>[2x]MSLAKNIVFIGFMGSGKSTLARALAKDLDLVFLDSDFLIEQKFNQKVSEIFEQKRENFFR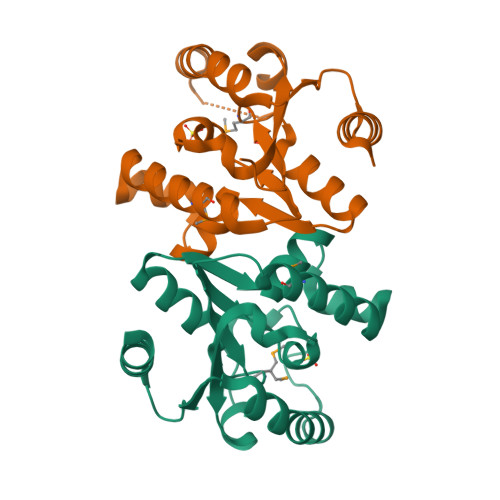EQEQKMADFFSSCEKACIATGGGFVNVSNLEKAGFCIYLKADFEYLKKRLDKDEISKRPLFYDEIKAKKLYNERLSKYEQKANFILNIENKNIDELLSEIKKVIKEGGSHHHHHH The principal CPS of the human pathogen and Tier 1 select agent Burkholderia pseudomallei consists of a linear repeat of –­3)-­2-O-acetyl-6-deoxy-β-d-manno-heptopyranose-(1–. This CPS is critical to the virulence of this emerging pathogen and represents a key target for the development of novel therapeutics. wcbI is one of several genes in the CPS biosynthetic cluster whose deletion leads to significant attenuation of the pathogen; unlike most others, it has no homologues of known function and no detectable sequence similarity to any protein with an extant structure. The structure revealed that WcbI adopts a predominantly helical fold: the N-terminal 100 amino acids form a ligand-binding domain fold, with the remaining 210 amino acids adopting an entirely novel fold. Based on the structure and on biochemical and biophysical data, we propose that WcbI functions as an acetyltransferase and requires another functional module to carry out this function.

The crystal structure of WcbI was determined by the multiple-wavelength anomalous dispersion method, using data collected at four wavelengths. No radiation damage to the crystal was apparent after the first three data sets, so the exposure times were increased for the low-energy remote data set, which was collected over an interval of 360° to a high resolution of 1.56 Å. The coordinates of 24 Br ions were used for phasing. The high resolution of the low-energy remote data set was crucial for subsequent density modification and successful building of the WcbI polyalanine model (605 residues out of 622) by SHELXE. For the correct hand, the correlation for the partial structure against the native data was 36.5%.1 The full WcbI atomic model was built by ARP/wARP using the polyalanine model produced by SHELXE and the low-energy remote data. This was found to contain bound CoA, carried through purification from the expression host, and will henceforth be termed the WcbI native structure. The structure of the CoA complex of WcbI and the native structure were refined by PHENIX and CCP4, respectively, to resolutions of 1.38 and 1.56 Å, respectively. The native structure contains 38 bromide ions. Interestingly, in the native structure the CoA terminal SH group points away from Cys14 toward Cys41, perhaps owing to a more reducing environment of the crystallization conditions. The two structures of WcbI presented here, obtained under different conditions, suggest that WcbI allows some flexibility in the CoA head group.

>[2x]SMAQRKKYSVYGSCQAPALAKMLNSCPTFARDWELVEMEPCFVASEEQIDRHLAETIPKLDLFLYQPVSEGYRGEKYSSVFLRNSMPPGGNALSVQYMHWEGYHPTVNSPYGLPPHPEGYVDALIAGAVVMDVDKETYLRHLEEIGASLRIDIDEIESWCVDELKTREVGENDGGKQIDISVTDFILANCRQKRLFYTMNHPTAALMREIAARCMLALGYTYSDISFDQNLDPLDVTKMSLYPIYRDCFDFSELNRMNEYQVLYKKKAYEPYLLEQFEWFERSPKADVSAFFDRVAANRRWVRTALRRAFES> GPLGSMAASGLDHLKNGYRRRFCRPSRARDINTEQGQNVLEILQDCFEEKSLANDFSTNSTKSVPNSTRKIK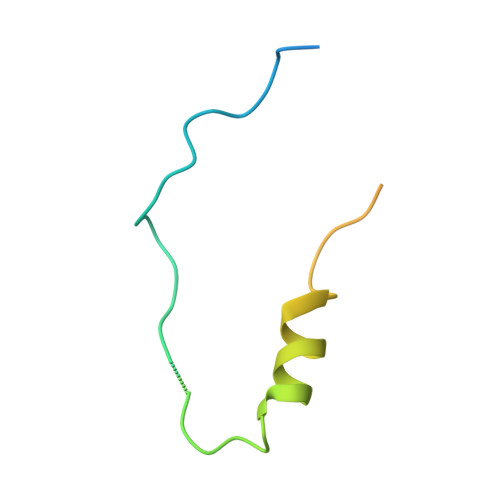DTCI>MHHHHHHLPNITILATGGSIAGGGDSATKSNYTVGKVGVENLVNAVPQLKDIANVKGEQVVNIGSQDMNDNVWLTLAKKINTDCDKTDGFVITHGSDTMEETAYFLDLTVKCDKPVVMVGAMRPSTSMSADGPFNLYNAVVTAADKASANRGVLVVMNDTVLDGRDVTKTNTTDVATFKSVNYGPLGYIHNGKIDYQRTPARKHTSDTPFDVSKLNELPKVGIVYNYANASDLPAKALVDAGYDGIVSAGVGNGNLYKSVFDTLATAAKTGTAVVRSSRVPTGATTQDAEVDDA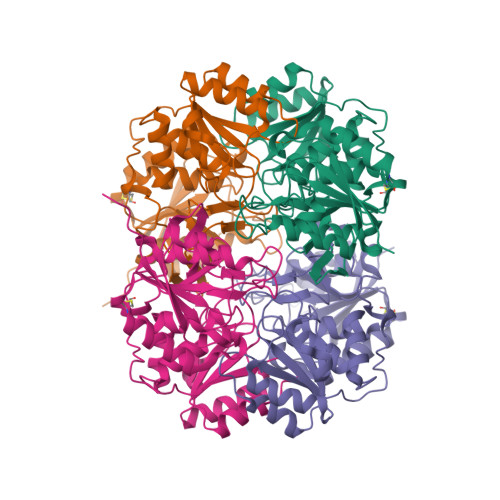KYGFVASGTLNPQKARVLLQLALTQTKDPQQIQQIFNQY[4x]>[2x]MTAIAPVITIDGPSGAGKGTLCKAMAEALQWHLLDSGAIYRVLALAALHHHVDVASEDALVPLASHLDVRFVSTNGNLEVILEGEDVSGEIRTQEVANAASQVAAFPRVREALLRRQRAF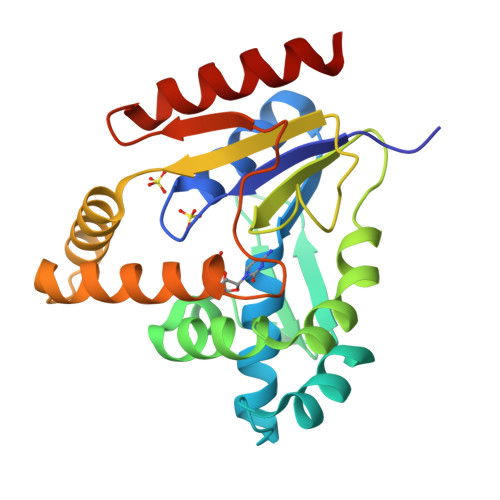RELPGLIADGRDMGTVVFPDAPVKIFLDASSEERAHRRMLQLQEKGFSVNFERLLAEIKERDDRDRNRAVAPLVPAADALVLDSTTLSIEQVIEKALQYARQKLALA>MYGLVNKAIQDMISKHHGEDTWEAIKQKAGLEDIDFFVGMEAYSDDVTYHLVGAASEVLGKPAEEWLIAFGEYWVTYTSEEGYGELLASAGDSLPEFMENLDNLHARVGLSFPQLRPPAFECQHTSSKSMELHYQSTRCGLAPMVLGLLHGLGKRFQTKV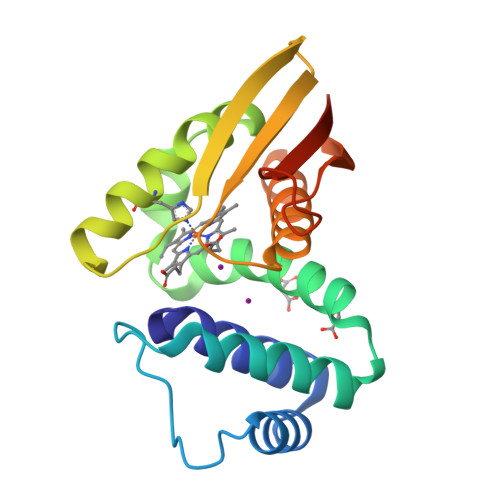EVTQTAFRETGEDHDIFSIKYEDSNLYDD[2x]The RNA recognition motif (RRM) binds to nucleic acids as well as proteins. Here we describe the mode of interaction between hnRNP L and LL with the methyltransferase SETD2. We demonstrate that for the interaction to occur, a leucine pair within a highly conserved stretch of SETD2 insert their side chains in hydrophobic pockets formed by hnRNP L RRM2. Notably, the SETD2 binding region in RRM2 is distinct from its RNA-binding interface.

HnRNP LL has a very similar amino acid sequence with 68% sequence identity and domain organization to its paralog hnRNP L. Immunoblotting of the purified complexes with anti-SETD2 and anti-HA antibodies demonstrated that similar to hnRNP L, the RRM2 of hnRNP LL interacts with SETD2. The ITC result showed that hnRNP LL binds to SETD22167–2192 with a mean KD value of 8.27 ± 0.28 μM, which is slightly weaker than that of hnRNP L (higher KD value suggests lower binding affinity). In the sequence alignment of RRM2 of hnRNP L vs. LL, we noted that the residues belonging to the SETD2 binding surface are highly conserved, except that I214 of hnRNP L corresponds to a Val in hnRNP LL. Next, we generated a hnRNP LLV188I mutant and performed ITC and found that it shows nearly the same binding affinity with SETD22167–2192 as that of hnRNP L. We next tried to crystallize the hnRNP LL RRM2–SETD22167–2192 complex but did not succeed. However, we got a high-resolution structure when a truncated peptide encompassing the core interacting motif of SETD2 2180SNPNAGKVLLPTP2192 was used for crystallization. We determined the structure in the P1 space group at a 1.60 Å resolution, with two almost similar hnRNP LL RRM2-SETD22180–2192 complexes in each crystallographic asymmetric unit. HnRNP LL-SETD22180–2192 structure shows high similarity to the structure of hnRNP L- SETD22167-2192complex (RMSD = 0.672 Å over 92 aligned Cα atoms). Similar results were observed when the binding of hnRNP LL RRM2 with SETD22180–2192 was tested and found to be weaker as compared to binding with SETD22167–2192.

>[2x]HHHHHHMNKVLLLSIQNPLYPITVDVLYTVCNPVGKVQRIVIFKRNGIQAMVEFESVLCAQKAKAALNGADIYAGCCTLKIEYARPTRLNVIRNDNDSWDYTKPYLGRRD;>SNPNAGKVLLPTP[2x]>GSHMAPLKDVYK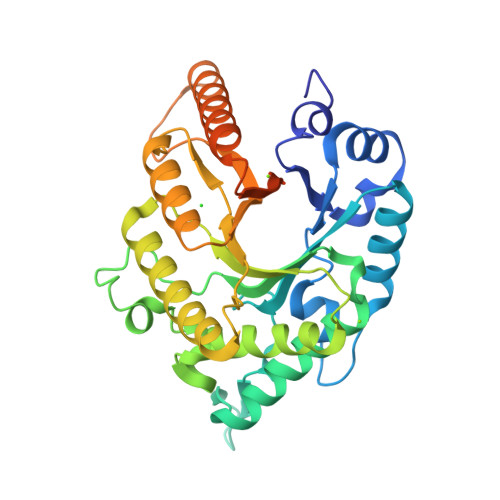NDFLIGNAISAEDLEGTRLELLKMHHDVVTAGNAMKPDALQPTKGNFTFTAADAMIDKVLAEGMKMHGHVLVWHQQSPAWLNTKKDDNNNTVPLGRDEALDNLRTHIQTVMKHFGNKVISWDVVNEAMNDNPSNPADYKASLRQTPWYQAIGSDYVEQAFLAAREVLDENPSWNIKLYYNDYNEDNQNKATAIYNMVKDINDRYAAAHNGKLLIDGVGMQGHYNINTNPDNVKLSLEKFISLGVEVSVSELDVTAGNNYTLPENLAVGQAYLYAQLFKLYKEHADHIARVTFWGMDDNTSWRAENNPLLFDKNLQAKPAYYGVIDPAEQ[8x]> GGGGUUAUGUGUGCCCGGCAUGGGUGCAGUCUAUAGGGUGAGAGUCCCGAACUGUGAAGGCAGAAGUAACAGUUAGCCUAACGCAAGGGUGUCCGUGGCGACAUGGAAUCUGAAGGAAGCGGACGGCAAACCUUCGGUCUGAGGAACACGAACUUCAUAUGAGGCUAGGUAUCAAUGGAUGAGUUUGCAUAACAAAACAAAGUCCUUUCUGCCAAAGUUGGUACAGAGUAAAUGAAGCAGAUUGAUGAAGGGAAAGACUGCAUUCUUACCCGGGGAGGUCUGGAAACAGAAGUCAGGAGAAGUCAUAGUACCCUGUUCGCAGGGGAAGGACGGAACAAGUAUGGCGUUCGCGCCUAAGCUUGAACGGCCGUAUACCGAACGGUACGUACGGUCGUGUG

Group II introns are ubiquitous self-splicing ribozymes and retrotransposable elements evolutionarily and chemically related to the eukaryotic spliceosome, with potential applications as gene-editing tools. The site also harbors a metal-ion cluster formed by two divalent (M1–M2) and two monovalent (K1–K2) ions. In the first step of splicing, depending on whether the intron follows a hydrolytic or a transesterification mechanism, respectively, a water molecule or the 2′-OH group of a bulged adenosine in D6, activated by M2 and by the triple helix, attack the 5′-splice junction of the precursor (5e-I-3e), forming an intron/3′-exon intermediate (I-3e), in which the scissile phosphate (SP) is coordinated by K2. In the second step of splicing, the 5′-exon (5e), activated by M1, performs a nucleophilic attack on the 3′-splice junction, releasing ligated exons (5e-3e) and a linear or lariat form of the excised intron.

After incorporating the resulting triple base mutations (C289A/C358A/G385U, aka the A-mutant; C289G/C358G/G385C, aka the G-mutant; and C289U/C358U/G385A, aka the U-mutant), we monitored effects on splicing kinetics. We then determined the crystal structures of the G and U mutants in the presence of sodium and magnesium at 3.2 and 3.3 Å resolution, respectively. However, the detailed architecture of the active site differs significantly from wild type under sodium conditions. By contrast with wild type, the G and U mutants in sodium maintain the triple helix configuration, as revealed by the Fo − Fc maps calculated by omitting the J2/3 residues and the catalytic metals (total peak height for the triple helix conformer of the G288 nucleobase = 7.5 σ in the G-mutant and = 9.3 σ in the U-mutant). Therefore, these structures show that the G and U mutants are unable to adopt the toggled conformation, which may explain their tendency to stall after the first step of splicing. Specifically, in the presence of near-physiological potassium and magnesium concentrations, the first splicing step of the G-mutant is ~12-fold slower and that of the U-mutant ~7-fold slower than in wild type. Moreover, the second splicing step of the G-mutant is ~48-fold slower and that of the U-mutant ~8-fold slower than in wild type. Most remarkably, both G and U mutants show accumulation of linear I-3e intermediate, which indicates that these mutants stall after the first step of splicing and have difficulty progressing into the second step. The release of K1 breaks the catalytic triple helix, and the intron begins sampling the toggled conformation. Such a rearrangement is significantly favored by protonation of N3C358, and it does not occur in the G and U mutants, which cannot be protonated.4-[({[(1R,2R,5R)-6,6-dimethylbicyclo[3.1.1]heptan-2-yl]methyl}amino)methyl]-N-hydroxybenzamide 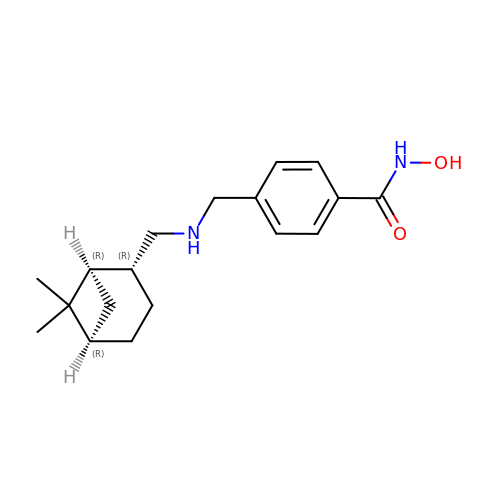| C18 H26 N2 O2 | JDQKGQWEIJPQSI-ARFHVFGLSA-N Bacteria usually express two highly conserved type IIA topoisomerases (Top2As), topoisomerase (topo) IV and DNA gyrase, involved respectively in chromosome relaxation/segregation and DNA supercoiling. Topo IV is a tetramer composed of two subunits, ParC and ParE, that form an active E2C2 complex; likewise gyrase through GyrA and GyrB subunits. Topo2As introduce a transient 4 bp staggered break into one DNA duplex and pass a second DNA duplex through the break which is then resealed. In this study, we have co-crystallized the ParE ATPase domain with short DNA duplexes in the presence of adenosine 5'-[β,γ-imido]triphosphate Adenylyl-imidodiphosphate (AMP-PNP), a non-hydrolysable ATP analogue that induces dimerization of ATPase domains to close the ATPase gate.

We report the first co-crystal structure of a topoisomerase ATPase complex with T-segment DNA captured inside a cavity formed by the protein dimer. Two ParE44 dimers were present in the asymmetric unit (AU): one dimer had a trapped T-segment DNA duplex in its central cylindrical hole (with evidence of weaker hole-bound density in the second dimer, likely washed out by the two possible alternative binding modes of the palindromic DNA to the second protein dimer). The 14-mer DNA duplex penetrates through the 22 Å hole in the protein formed by the ParE44 RNAse P-like domains and is mainly in the B form apart from a kinked region between basepairs 3 and 4 (i.e., between the first two AT and TA basepairs after the 5’-terminal GC and CG pairs). The DNA experiences in total a complex and asymmetric 39.4° change of direction. The major and minor grooves of the duplex are oriented towards opposite RNAse P-like domains of the ParE44 dimer and are almost equalized in width due to kinking. The protein-interacting 6 bp segment of the 14-mer duplex DNA, 5′-GCATAT is asymmetrically bounded by the RNAse P-like domains comprising an upper arch formed by protein residues in the region 269–291 and by the short helices comprising residues 316–322 at the end of the anti-parallel β-sheet which also in turn binds in the major and minor grooves of the double helix from both sides of the dimer. The structure reveals that one DNA end is bound in the ParE hole and is bent; the other 5′-GCATAT DNA end is not bound to protein, protrudes into solvent, adopts a B-form helix and is unbent. Interestingly, the DNA is bound asymmetrically in the hole. Thus, the top strand (asterisked in Fig. 2a, d) is bound by residues derived uniquely from one or other RNAse P-like domain in the dimer (but not both), in contrast to the more symmetric engagement of the bottom DNA strand (double asterisk) by pairs of residues S268, R396 and R400 contributed by both subunits. Interestingly, the ParE ATPase region introduces a kink into the T-segment DNA inducing a 40° bend, and moreover binds the DNA asymmetrically in the cavity through differential interactions with charged protein residues lining the hole.

>AMSKKEININNYNDDAIQVLEGLDAVRKRPGMYIGSTDGAGLHHLVWEIVDNAVDEALSGFGDRIDVTINKDGSLTVQDHGRGMPTGMHAMGIPTVEVIFTILHAGGKFGQGGYKTSGGLHGVGSSVVNALSSWLEVEITRDGAVYKQRFENGGKPVTTLKKIGTAPKSKTGTKVTFMPDATIFSTTDFKYNTISERLNESAFLLKNVTLSLTDKRTDEAIEFHYENGVQDFVSYLNEDKEILTPVLYFEGEDNGFQVEVALQYNDGFSDNILSFVNNVRTKDGGTHETGLKSAITKVMNDYARKTGLLKEKDKNLEGSDYREGLAAVLSILVPEEHLQFEGQTKDKLGSPLARPVVDGIVADKLTFFLMENGELASNLIRKAIKARDAREAARKARDESRNGHHHHHH[4x]>[2x]MEKRMSTQQRAAGNACPTAAFSFDPARLAQRRRWAGAFAALCGLALSPSALLAEEHSQHQDH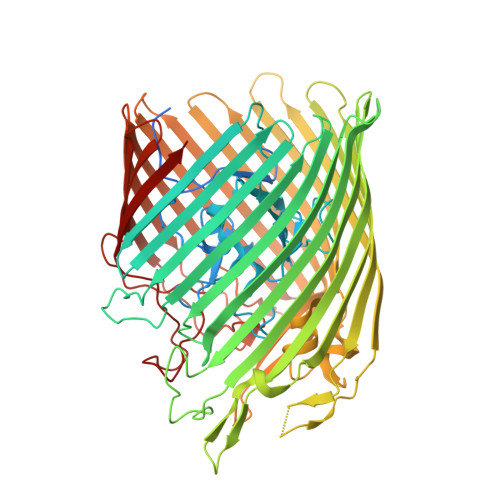AVELAPSVVTGVAQSSPLTIVTNPKEPRQPVPASDGADYLKTIPGFAVIRNGGSNGDPVLRGMFGSRLNILTNGGMMLGACPNRMDAPTSYISPETYDKLTVIKGPQTVLWGPGASAGTILFEREPERFGELGSRVNASLLAGSNGRFDKVLDAAAGNRLGYLRFTGNHAQSDDYEDGAGNTVPSRWKKWNGDVAVGWTPDEDTLIELTAGKGDGEARYAGRGMDGSQFKRESLGLRFVKSNVSDVLEKVEAQVYYNYADHIMDNFRLRTPDPSSMMPMPMASQVDRRTLGGRLAATWRWDDFKLVTGVDAMRNEHRARGSKYDMMTDYYTDADQFPWSKDAVFHNYGAFGELTWFAAERDRLIGGLRLDRASVKDYRQTLKSGHMGHAMANPTANDTRADTLPSGFVRYEHDLADSPTTLYAGLGHAERFPDYWELFSPKRGPNGSVNAFDKIKPEKTTQLDFGLQYNGDKLQAWASGYVGVVQDFILFSYREGMMGSSTQATNVDARIMGGELGASYQLTGNWKTDASLAYAWGKNSSDDRALPQIPPLEARFGLTYEEGDWSAGSLWRVVAPQNRIARDQGNVVGKDFDKSAGFGVFSLNGAYRVTRNVKLSAGVDNLFDKDYTEHLNKAGDAGFGFSANETVPEPGRTFWTKVDFSF> GGLGLIKSLAEKEKQLLERLEAAKKEAEERVKRAEAEAKALLEE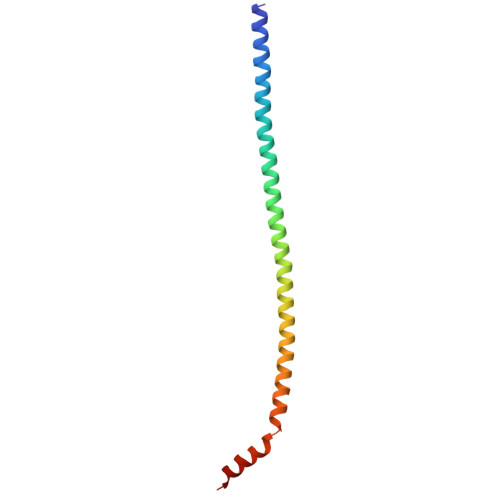AEAKAKALEAQYRERERAETEALLARYRERAEAEAKAVREKAMARLDEAVALVLKEVLP>MKQYLELMQKVLDEGTQKNDRTGTGTLSIFGHQMRFNLQDGFPLVTTKRCHLRSIIHELLWFLQGDTNIAYLHENNVTIWDEWADENGDLGPVYGKQWRAWPTPDGRHIDQITTVLNQLKNDPDSRRIIVSAWNVGELD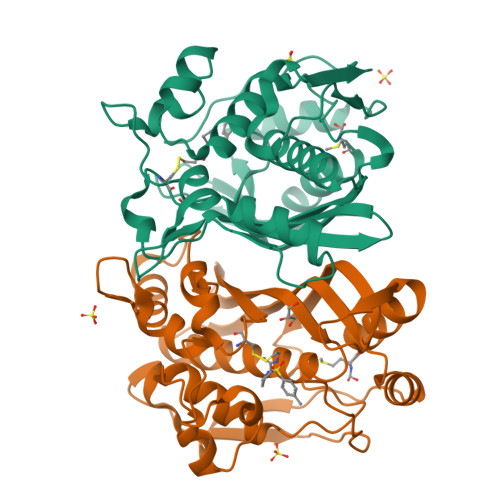KMACAPSHAFFQFYVADGKLSCQLYQRSCDVFLGLPFNIASYALLVHMMAQQCDLEVGDFVWTGGDTHLYSNHMDQTHLQLSREPRPLPKLIIKRKPESIFDYRFEDFEIEGYDPHPGIKAPVAI[2x]> GSRVAILWHEMWHEGLEEASRLYFGERNVKGMFEVLEPLHAMMERGPQTLKETSFNQAYGRDLMEAQEWCRKYMKSGNVKDL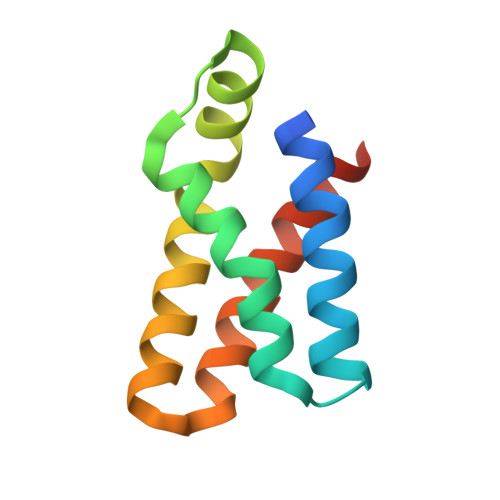TQAWDLYYHVFRRISKQSGG D-ALANINE | C3 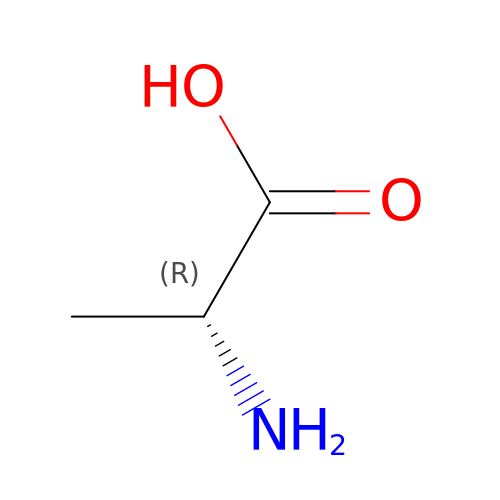H7 N O2 | QNAYBMKLOCPYGJ-UWTATZPHSA-N5-(2-amino-1,3-thiazol-4-yl)-2-chlorobenzene-1-sulfonamide | C9 H8 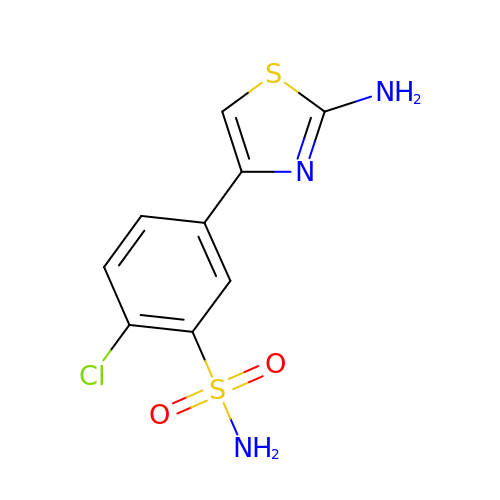Cl N3 O2 S2 | YZFWRSMMUCDYLX-UHFFFAOYSA-N> HHHHHHGSGTDRLKGKVAIVTGGTLGIGLAIADKFVEEGAKVVITGRHADVGEKAAKSIGGTDVIRFVQHDASDEAGWTKLFDTTEEAFGPVTTVVNNAGIAVSKSVEDTTTEEWRKLLSVNLDGVFFGTRLGIQRMKNKGLGASIINMSSIEGFVGDPTL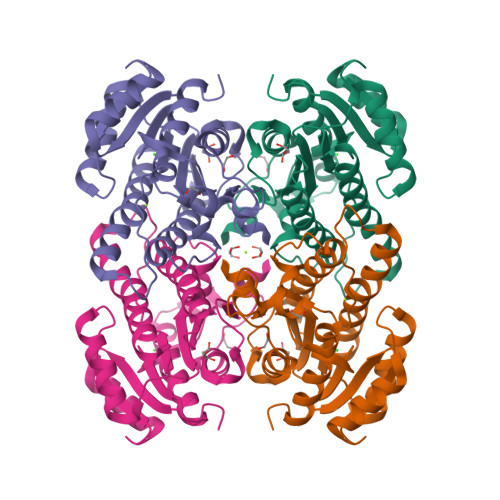GAYNASKGAVRIMSKSAALDCALKDYDVRVNTVHPGYIKTPLVDDLEGAEEMMSQRTKTPMGHIGEPNDIAWICVYLASDESKFATGAEFVVDGGYTAQ>[6x]GSHMKPEIKEAYMKTAELFSQVSNCKRMKVGAIVVKNGSILA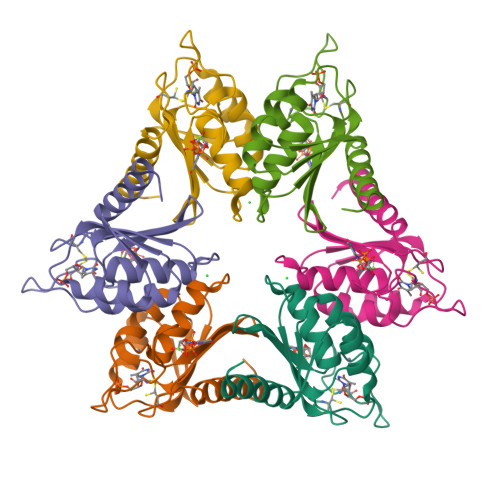HGWNGTPSGFHTNCCELEDGSTNPFVLHAEQNALVKMAKSSESIDGSELFCTHSPCPDCSKMIAQAGVKKVYYRNEYRITDGIDVLQQLGVEVEKM> SSLHIAMFPWFAMGHLIPYLHLSNKLAKRGHKISFFTPKKTQTKLEQFNLYPNLITFYPLNVPHVDGLPFGAETTSDVAISLGPILMTAMDQTQNQIELLLTQLKPQI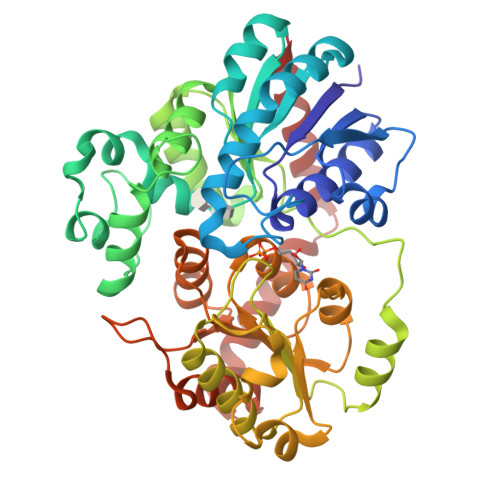IFFDFVFWLPKITQRLGIKSFLYFIINPATISYTTSPPRMFEAENLTEVDLMKPPKGYPTSFNLQSHEAKHLASTRKIEFGSGIPFSVRSYNCLSLTDAIGFKGCREIEGPYVDYLQEQFGKPVLLSGPVLPEQSKTALDEKWGSWLGGFKDGSLVYCALGSELKLKQDQFHELLLGLELTGFPFLAILKPPVGFETIEDALPEGFKERVKEKGIVHSGWIQQQLILEHPSVGCFVTHCGAGSITEGLVNNCQMVLLPQLNGDYIINARIMGRHLKVGVEVKKGEEDGLFTKESVYEAVKIVMDDENEIGREVRSNHTKVRNLLLRHDLESSCLDTFCEKLQELVS> GYSDRARSITLGNSTITTQECANVVVGYGVWPDYLKDSEATAEDQPTQPDVATCRFYTL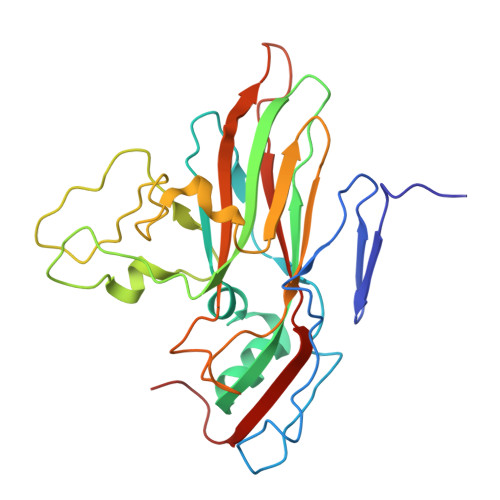DSVQWQKTSPGWWWKLPDALSNLGLFGQNMQYHYLGRTGYTVHVQCNASKFHQGCLLVVCVPEAEMGCATLDNTPSSAELLGGDSAKEFADKPVASGSNKLVQRVVYNAGMGVGVGNLTIFPHQWINLRTNNSATIVMPYTNSVPMDNMFRHNNVTLMVIPFVPLDYCPGSTTYVPITVTIAPMCAEYNGLRLAGHQ3-(2-amino-5-chloro-1H-benzimidazol-1-yl)propan-1-ol | C10 H12 Cl N3 O | 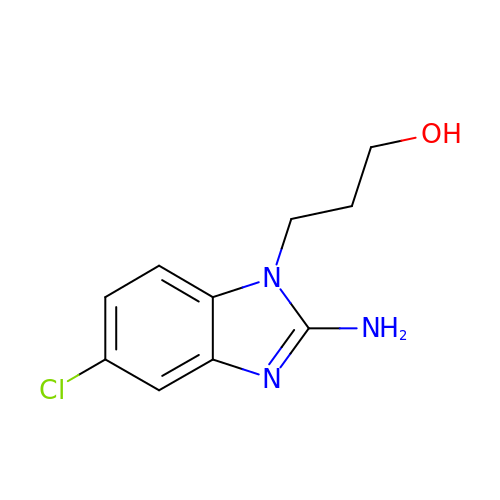NSMVCZCLMLZSOB-UHFFFAOYSA-N>SNAMNVYTFDFNDIKNQSDFYR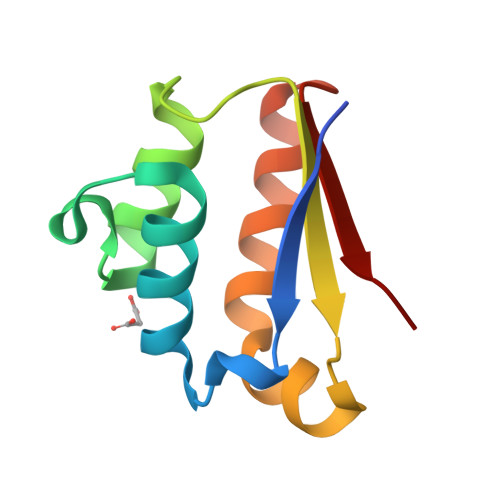EFTQTFGLASEKVSDLDTLWDAVMSDILPLPLEIEFVHLPDKLRRRYGALILLFDEAEEELEGRLRFNVRH[2x]(3R)-3-(3-chlorophenyl)-3-[(5-methyl-7-oxo-6,7-dihydro[1,2,4]triazolo[1,5-a]pyrimidin-2-yl)amino]propanenitrile 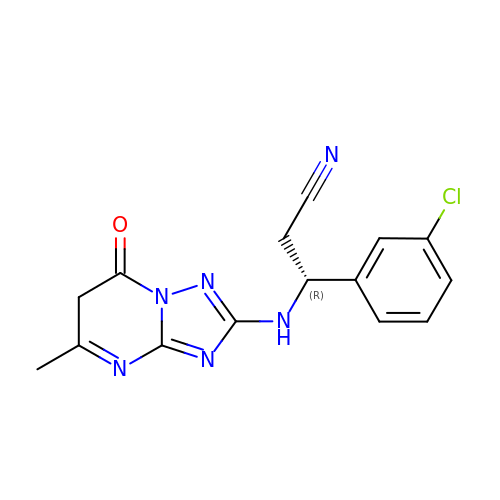| C15 H13 Cl N6 O | NHMPMHHRMRFBHQ-GFCCVEGCSA-N> MVKKPPKSYDEYKQVDVGKDGMVATAHPLASEIGADVLKKGGNAIDAAVAIQFALNVTEPMMSGIGGGGFMMVYDGKTKDTTIIDSRERAPAGATPDMFLDENGKAIPFSERVTKGTAVGVPGTLKGLEEAL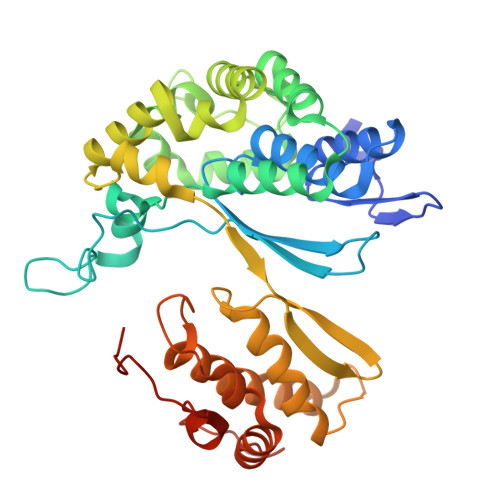DKWGTRSMKQLITPSIKLAEKGFPIDSVLAEAISDYQEKLSRTAAKDVFLPNGEPLKEGDTLIQKDLAKTFKLIRSKGTDAFYKGKFAKTLSDTVQDFGGSMTEKDLENYDITIDEPIWGDYQGYQIATTPPPSSGGIFLLQMPKILDHFNLSQYDVRSWEKYQLLAETMHLSYADRASYAGDPEFVNVPLKGLLHPDYIKERQQLINLDQVNKKPKAGDPWKYQEGSANYKQVEQPKDKVEGQ>ASWSHPQFEKGALEVLFQGPGDPIHGHIELHPLLVRIIDTPQFQRLRYIKQLGGGYYVFPGASHNRFEHSLGVGYLAGCLVHALGEKQPELQISERDVLCVQIAGLCHDLGHGPFSHMFDGRFIPLARPEVKWTHEQGSVMMFEHLINSNGIKPVMEQYGLIPEEDICFIKEQIVGPLESPVEDSLWPYKGRPENKSFLYEIVSNKRNGIDVDKWDYFA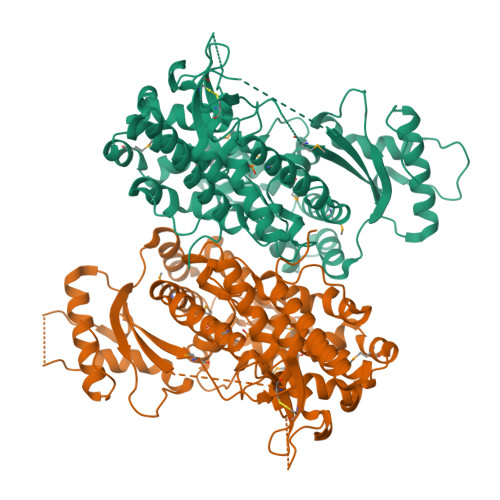RDCHHLGIQNNFDYKRFIKFARVCEVDNELRICARDKEVGNLYDMFHTRNSLHRRAYQHKVGNIIDTMITDAFLKADDYIEITGAGGKKYRISTAIDDMEAYTKLTDNIFLEILYSTDPKLKDAREILKQIEYRNLFKYVGETQPTGQIKIKREDYESLPKEVASAKPKVLLDVKLKAEDFIVDVINMDYGMQEKNPIDHVSFYCKTAPNRAIRITKNQVSQLLPEKFAEQLIRVYCKKVDRKSLYAARQYFVQWCADRNFTKPQDGDVIAPLITPQKKEWNDSTSVQNPTRLREASKSRVQLFKDDPM[4x]>[2x]GSHMRKYDVSLTPSGIKVNDEITLLYPALKYAEELYLLINQNKINFIKSMAWPAFVNNISDSVSFIEQSMIDNQNEKALILFIKYKTKIAGVVSFNIIDHANKTAYIGY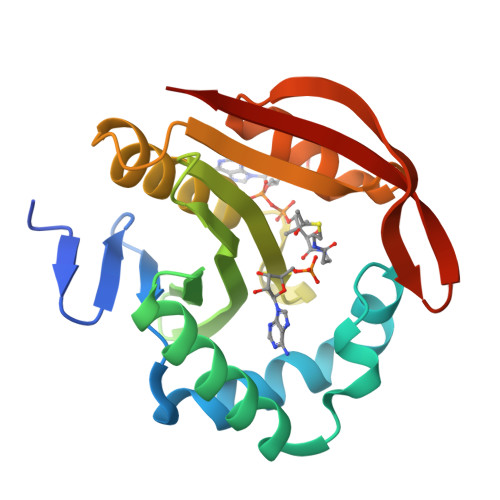WLGANFQGKGIVTNAINKLIQEYGDSGVIKRFVIKCIVDNKKSNATALRCGFTLEGVLQKAEILNGVSYDQNIYSKVIG[2-[[(2S)-1-[bis(phenylmethyl)amino]-5-[[N-(methylcarbamoyl)carbamimidoyl]amino]-1-oxidanylidene-pentan-2-yl]amino]-2-oxidanylidene-ethyl]-diazonio-azanide 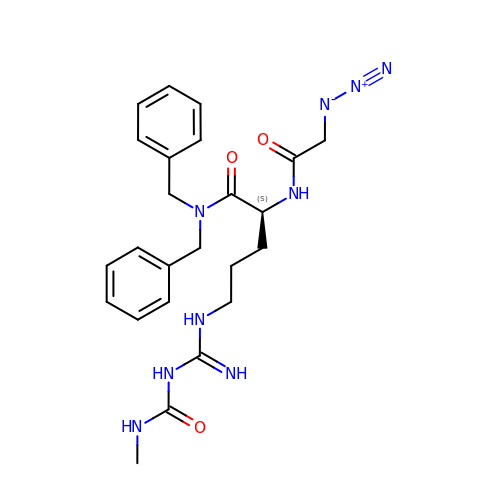| C24 H31 N9 O3 | WCLXSHAWFUUDKF-FQEVSTJZSA-N More specifically, the imidazole ring of the substrate is hydrolytically opened with the assistance of an essential zinc ion, and the resulting pyrimidine intermediate undergoes an Amadori rearrangement of the carbohydrate side chain followed by ring closure. The enzyme product, dihydroneopterin triphosphate, serves as the first committed intermediate in the biosynthesis of tetrahydro­folate by many microorganisms and as the first committed intermediate in the biosynthesis of tetrahydro­biopterin by animals.

Equilibrium sedimentation yielded a molecular weight of 212 ± 30 kDa. Boundary sedimentation resulted in a sedimentation velocity of 9.6 S. Mass spectrometry revealed the presence of 0.9 moles of zinc per mole of polypeptide. The r.m.s.d. values to previously reported GTP cyclohydrolase I structures were in the range 0.76–1.3 Å for the monomers, whereas r.m.s.d. values in the range 0.12–0.34 Å were found on comparing individual L. monocytogenes GTP cyclohydrolase I monomers. However, no appreciable density representing the essential zinc ions was present, and the two canonical cysteine residues Cys78 and Cys150 that form part of the putative zinc-binding site (for a sequence alignment) were oxidized to the disulfide level; it is most probable that the zinc had been lost owing to the chelating activity of the citrate that was used as a precipitant, and loss of the metal cation had been followed by oxidation of the zinc-chelating cysteine residues. A similar observation had previously been made for crystals of GTP cyclohydrolase I from E. coli that had been exposed to EDTA. In comparison, the Listeria protein appears to be even more sensitive to chelator-induced zinc-ion loss, but a search for other (nonchelating) crystallization conditions has been unsuccessful to date. The residues lining the active-site cavity of the L. monocytogenes protein have high temperature factors, possibly owing to the absence of a divalent cation. The enzyme from L. monocytogenes is similar in terms of sequence and three-dimensional structure to orthologs from eubacteria (E. coli and Yersinia pestis). The structure is also similar to mammalian cyclohydrolase I (rat and mouse), although the mammalian protomers are somewhat longer. Semilogarithmic dose–response curves showed symmetrical, S-shaped features, and the overall Z factor of the screen was 0.87. Three heterocyclic compounds inhibited the L. monocytogenes enzyme with IC50 values in the low double-digit micromolar range while not acting as strong inhibitors of human GTP cyclohydrolase I (for details of the high-throughput assay, see the supporting information).

>[10x]MHHHHHHGSDDDDKEQIDKQKIADAVKVILEAVGENPDREGLIDTPMRVARMYEEVFAGLKKDPSVHFDTIFEEQHEELVLVKDIRFSSMCEHHLVPFFGVAHVAYLPQNGRVAGLSKLARVVDDVSRRPQLQERITTTVAEIMMEKLKPLGVMVIMEAEHMCMTIRGVNKPGTKTITSAVRGAFKNDDKLRSEVLALIKHN> MDKFRVQGPTRLQGEVTISGAKNAALPILFAALLAEEPVEIQNVPKLKDIDTTMKLLTQLGTKVERDGSVWIDASNVNNFSAPYDLVKTMRASIWALGPLVARFGQGQVSLPGGDAIGAAPVDLHIFGLEKLGAEIKLEEGYVKASVNGRLKGAHIVMDKVSV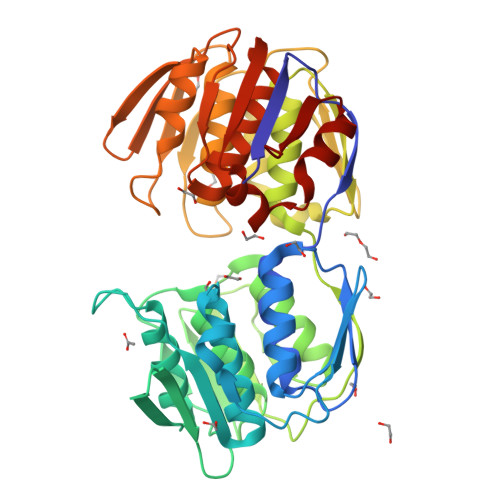GATVTIMSAATLAEGTTIIENAAREPEIVDTANFLVALGAKISGQGTDRITIEGVERLGGGVYRVLPDRIETGTFLVAAAISGGKIVCRNAQPDTLDAVLAKLREAGADIETGEDWISLDMHGKRPKAVTVRTAPHPAFPTDMQAQFTLLNLVAEGTGVITETIFENAFMHVPELIRMGAHAEIESNTVICHGVEKLSGAQVMATKLRASASLVLAGCIAEGTTVVDRIYHIDRGYERIEDKLRALGANIERVKGE> VEWTDKERSIISDIFSHMDYDDIGPKALSRCLIVYPWTQRHFSGFGNLYNAEAIIGNANVAAHGIKVLHGLDRGVKNMDNIAATYADLSTLHSEKLHVDPDNFKLLSDCITIVLAA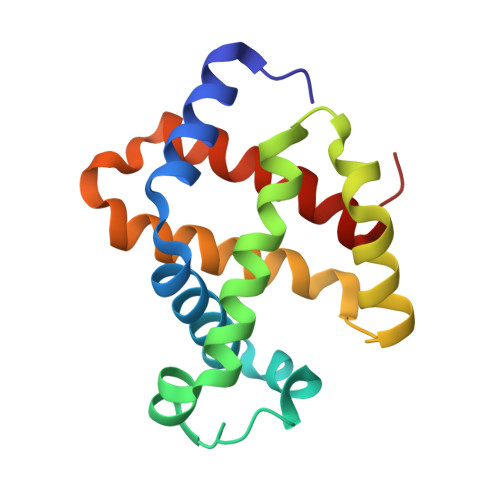KMGHAFTAETQGAFQKFLAVVVSALGKQYH>GTENLYFQSNAMKFKIHSDITYQVMSPTTFIFNVHALRTESQHILDESLIVTPPIEIEEFSYNSGTSRFVRLKATENTTFSMSYTATVDTQYKVIDQRQELETVPVVDLDGDIIPFLFPSRYCQSDKLQKLAYKEFGKIENVYSKVLAITDWIYNNVEYISGSTNSQTSAFDTITERAGVCRDFAHLGIALCRALSIPARYFTGYAFK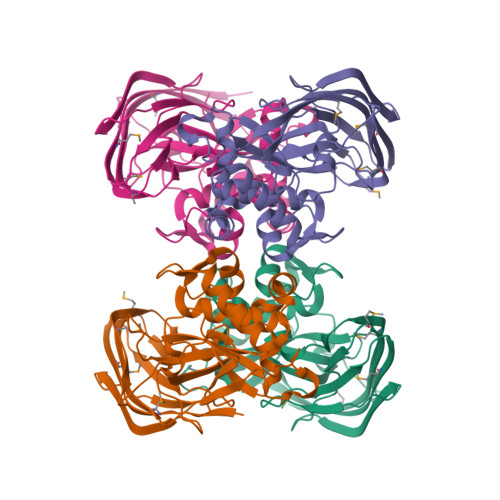LNPPDFHACFEAYIGGNWIIFDATRLVPLNGLVKIATGRDAADAAVASIFGNASSTNMHVECASLDTDFTPFWYDKNSLKGLSFQ[4x]>[2x]MRGSHHHHHHGSSHANINAFKEAVTKIDRVEINR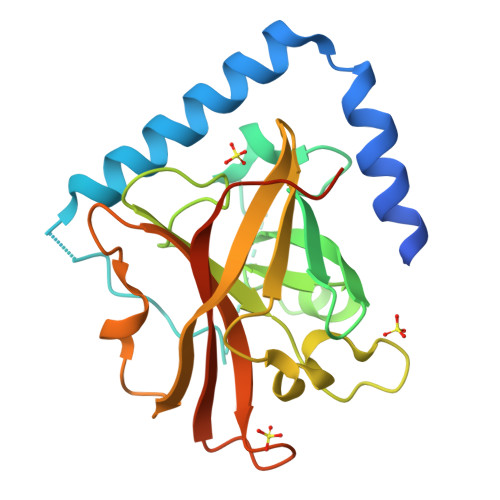RLELAYAYNASIAGAKTNGEYPALKDPYSAEQKQAGVVEYARMLEVKEQIGHVIIPRINQDIPIYAGSAEENLQRGVGHLEGTSLPVGGESTHAVLTAHRGLPTAKLFTNLDKVTVGDRFYIEHIGGKIAYQVDQIKVIAPDQLEDLYVIQGEDHVTLLTCTPYMINSHRLLVRGKRIPYVEKTVQKDSKTFRQQQ> MVVLAASICTRGGKAVLARAFHDIKRSRVEALLASFPKAANSGTQHTTVEQDNVRFVYQPLDELYMVLITNKQSNILQDIDTLHLFAQVVTNTCRTLEEREILRNAYELISAFDEIINLGYRENLTINQIKTFLEMESH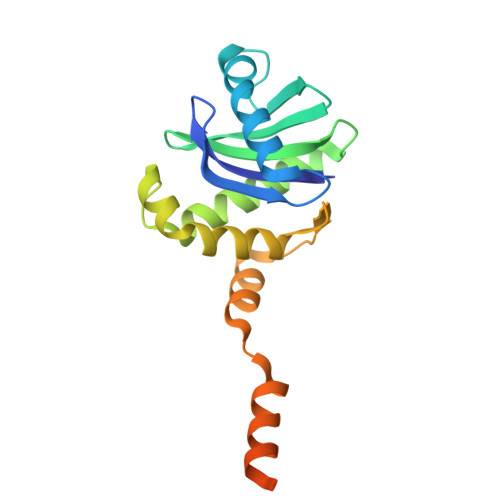EERIQEIIARNKELEATEERKRKAKQLEMQRKEASR>[2x]ADIIYQFHSFEDIIQLSESLQRIGITGGTVYHYDGQYFLSLE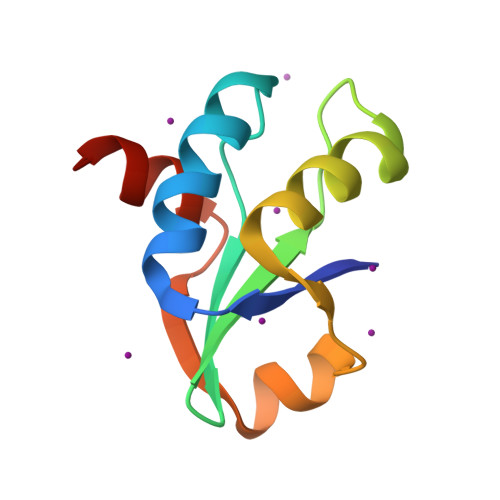DLGSHTAEGVVAVLAEYGNPTTLTIYRLQEYGKLIMDGNAVETIQTHFS> HMNATVETTQHDVEGTGAAGATAMLFPGMGPAAFSDVGRFMVTNRYTRELLAEADDTLGYSLVDRFRQAEGDYSEYAQIAFLVNCVALARWAEQTMDLTPRICAGACFGEKSVAAYSGALTFADAVRMTAGLARCMDEYF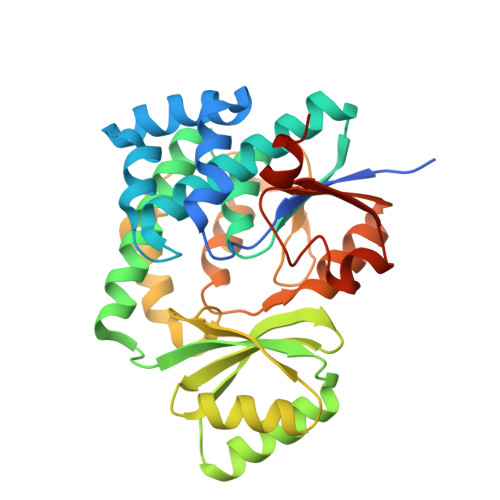RTEHLGVVTHSFVRAPRERLDEILAELDERGEWHEISCHIDHDFFMLTLHERNSVWLEGRLRSVGAMPLYAMRPPMHAAAFGGLRDKAEEEVIAPLTFHDPTLPVVADQDGKVLTTGDEVRTMLLESFVRPLRWPDVISSLQDQGVTRVCVAGPDSLFGRVGTTTRAFEVIAATPRLALQPRARTTSR Human 3-phosphoglycerate dehydrogenase (PHGDH) is responsible for the NAD+-dependent conversion of 3-phosphoglycerate (3-PG) to phosphohydroxypyruvate (PHP), which is the first step in the de novo serine synthesis pathway. Thus, PHGDH activity diverts glycolytic flux into biomass production. Limited proteolysis with thermolysin revealed a stable fragment of PHGDH consisting of the core of the catalytic domain containing the cofactor-binding site, and this was shown to crystallise readily. Thus PHGDH-93 provides a valuable tool to investigate binders to the cofactor-binding site.

PHGDH-93 was then successfully crystallised with an empty, accessible cofactor-binding pocket. Soaking of all 15 fragments into PHGDH-93 crystals was performed overnight at RT using a fragment concentration of 80 mM in 20 % DMSO. Difference electron density corresponding to seven fragments (3, 5, 9, 10, 14-16, 47 % of tested compounds) was clearly visible. All of the fragments for which crystallographic data were obtained bound to the adenine-pocket suggesting this pocket to be a preferential site for fragment binding. Analysis of the fragments’ binding modes showed that four of the fragments (5, 14, 15 and 16) were coordinated by hydrogen and/or halogen bonds, whereas the other three fragments (3, 9 and 10) appeared to be stabilised only by apolar contacts. Of the four compounds forming specific interactions with the protein, fragments 5 (3-chloro-4-fluorobenzamide), 14 (5-fluoro-2-methylbenzoic acid) and 15 (N-(3-chloro-4-methoxyphenyl)acetamide) constitute substituted benzene rings. Fragment 14 was substantially less potent (Kd = 26 ± 31 mM) compared to the two structurally similar fragments 5 and 15 (5, Kd = 1.6 ± 0.2 mM and 15, Kd = 2.8 ± 1.6 mM). However, fragment 14 still formed a hydrogen bond with the side-chain of Asp174 and a water molecule present in the binding pocket.

>[2x]MLVMNTPNGNSLSAAELTCGMIMCLARQIPQATASMKDGKWERKKFMGTELNGKTLGILGLGRIGREVATRMQSFGMKTIGYDPIISPEVSASFGVQQLPLEEIWPLCDFITVHTPLLPSTTGLLNDNTFAQCKKGVRVVNCARGGIVDEGALLRALQSGQCAGAALDVFTEEPPRDRALVDHENVISCPHLGASTKEAQSRCGEEIAVQFVDMVKGKSLTGV>[4x]MKAIPPKIWFETQLKGSGL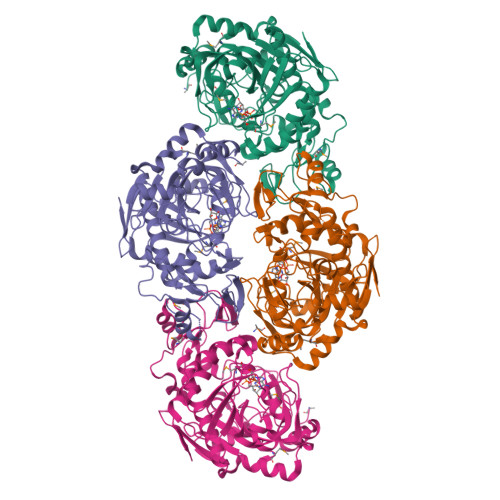DKKFQIDELIETQSSVRVFANKKYLPDTETINEALTKVTAVNVSGDKSGYFQNGLPFPNEAGYFEKIPVGHPELLSPIERLTGSKKIVSSHSLVTASGGYPLTNPLLPYRKPIRVSIFSLAGPSFENNYLHYRLFLLDSVQKIIDSPLFSHLHDGLPIQFDEAKKELGEYDTNKLMARIRLGFPYLARFSSGGFYPSFSKSNAIIFLSEAYFRYQLEDVSLLLASVNQTGKETGKAALLKATAVGMGFFAKIDCGYDIQHIIFPYYLRAYKKLLSEHKFPWIAKIEFPIFNEIQQEQFDSIFEDYDGPTKVYRSTRDVLEFREEEIEKYLPAAINPSDAFALTGNEWGYGSVESMIGNNSSIRFDQVHHMNPLILDPSHHVEAQINKDHGVELT> GAMGS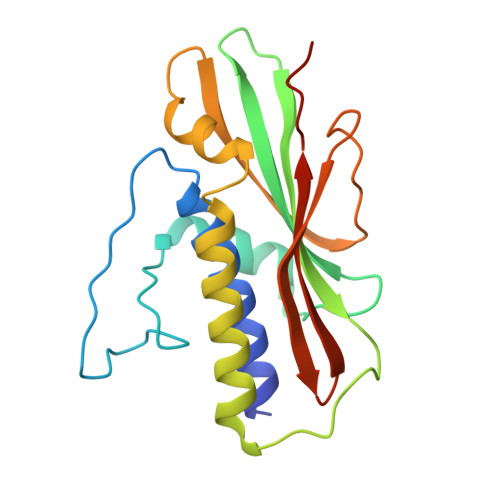DLDKFIKFFALKTVQVIVQARLGEKICTRSSSSPTGSDWFNLAIKDIPEVTHEAKKALAGQLPAVGRSMCVEISLKTSEGDSMELEIWCLEMNEKCDKEIKVSYTVYNRLSLLLKSLLAITRVTPAYRLSRKQGHEYVILYRIYFGEVQLSGLGEGFQTVRVGTVGTPVGTITLSCAYRINLAFMSTRQ> MKLAQGAFVDVIRIGALSPPTDQRSLWARTLLSEAVDQGLDSLPVPLQDVSTFTVTLQPALAVRLKALADQHNTPVSVYAAGLIEAMRRRSESGSVAEAPMELPADALPGEGAVREVLRPLLKQAAEKTAAGKIVFAEAATGTGKGRMIASLAAAAAIKGDTVVVSAPLAVTWQLVNDMKDIPEVRRVGLTLSLGRPNFISPQRTLEWAIDNERADLAAWIEGGGKPLSLRSMETSKVISHELCWLLEDALLLAEDLPADSLLLTSEDPADCPAQQLYVAMRSNYTEAGIILCSHFMLAAHTRMMQMRGLGNDEELDDEAPTGLSLPHFIDTLIVDEAHLLEQAFASVYTHTLRLRPLMRTIEGLGSRGRKPALDALKELFTQMQVASARSTNTSLNVPLSDVPELIPALKDTVKTLGALPTKGMSRDARSVIRIATRAANDALSGHSRLRIEVTPVHSYPMLLSGRSNLQRALLGLWNATGGATLVSATLFTTGDNGSLTRWKLEVPTERAAFLPPVHPAWTTAPVLLHKEFCAHEPDDSPEWATECAQTIQGVASTAQGGTLVLCTSYQNTELLAGRLGAALGDRLIVQSKTSSAATCLAQFKAKHKAGIRPVWLGLGAAWTGIDLSDHSLPDNPELDRLLSDLVITRIPVGQNRSLTHERRTAIGGFRIISQEAAWHFRQGLGRLVRRPGVTHKNLWVLDARIYGGAAWVAPFRQILDRYKKA

CasDinG is an ATP-dependent 5′-3′ DNA helicase essential for bacterial Type IV-A1 CRISPR associated immunity. To provide immunity against plasmids, it is proposed that type IV-A systems bind DNA with an RNA-guided multi-protein Csf complex, and then recruit an accessory helicase called CasDinG to the DNA. It is supposed that, once loaded onto Csf-complex-bound DNA, CasDinG uses its ATP-dependent 5′-3′ helicase activity to silence transcription of nearby genes, mediating immunity. CasDinG contains an essential N-terminal domain predicted to bind DNA.

In an attempt to determine the structure of the N-terminal domain we solved the structure of a new crystal form of Pa CasDinG where overhang dsDNA substrates were included in our crystal conditions. To test our hypothesis, we screened crystals of Pa CasDinG grown in the presence of a 5’-overhang duplex DNA substrate. Orthorhombic crystals grew from precipitate after two weeks. We found that Pa CasDinG in the crystals had been proteolyzed corresponding to a ~12 kDa shift in molecular weight. The diffraction pattern corresponded to a unit cell of 67.04 Å x 84.01 Å x 97.619 Å and a P 21 21 21 space group, distinct from the unit cells of previously solved crystal structures. Matthews probability coefficient suggested a single solution of 1 CasDinG subunit in the unit cell with a solvent content of 29.75%. This was in the bottom quartile of solvent content for this resolution range, suggesting that CasDinG was tightly packed in this crystal morphology. The structure of Pa CasDinG revealed two helicase domains (HD1 and HD2) and two accessory domains (FeS-like and Arch domains), that aligned well (RMSD = 0.547 Å) with other models of Apo Pa CasDinG. Consistent with our Urea-PAGE analysis, no density for nucleic acid was observed. Additionally, no density was observed for the N-terminal domain of Pa CasDinG, despite the tight crystal packing, which we had hoped would constrain the previously observed flexibility of the domain.>SSSHPIFHRGEFSVCDSVSVWVGDKTTATDIKGKEVMVLGEVNINNSVFKQYFFETKCRDPNPVDSGCRGIDSK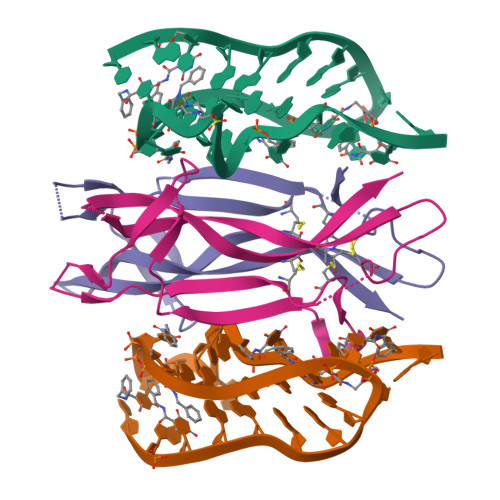HWNSYCTTTHTFVKALTMDGKQAAWRFIRIDTACVCVLSRKAVRRA[2x]> EA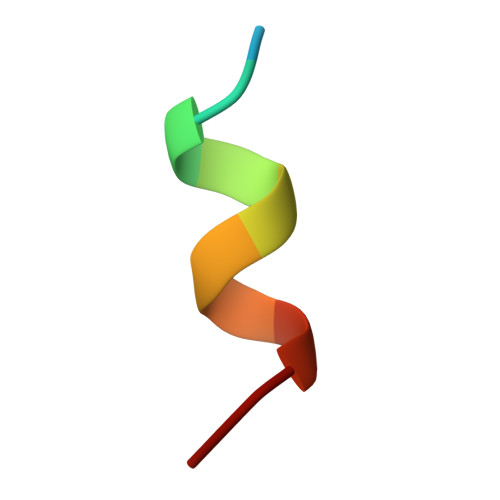LAGLSALFG> GTTKHSKLLILGSGPAGYTAAVYAARANLQPVLITGMEKGGQLTTTTEVENWPGDPNDLTGPLLMERMHEHATKFETEIIFDHINKVDLQNRPFRLNGDNGEYTCDALIIATGASARYLGLPSEEAFKGRGVSACATSDGFFYRNQKVAVIGGGNTAVEEALYLSNIASEVHLIHRRDGFRAEKILIKRLMDKVENGNIILHTNRTLEEVTGDQ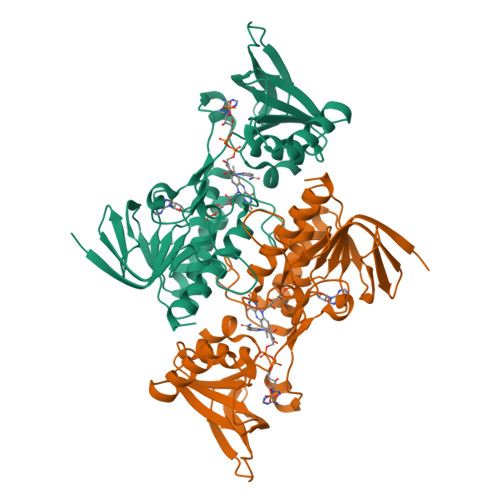MGVTGVRLRDTQNSDNIESLDVAGLFVAIGHSPNTAIFEGQLELENGYIKVQSGIHGNATQTSIPGVFAAGDVMDHIYRQAITSAGTGCMAALDAERYLDGL One family of these GEFs is comprised of the Ras guanine-nucleotide releasing proteins (RasGRPs) that can activate Ras or Rap, of which there are four in humans. GEFs activate Ras-family members by triggering the release of GDP and its replacement by GTP. The N-terminal portion of the RasGRPs contains the catalytic module that is common to other GEFs that operate on Ras-family members. This module consists of a Ras-exchanger motif (REM) domain followed by a Cdc25 domain. As first revealed by structural analysis of the Ras-specific GEF Son-of-Sevenless (SOS), the Cdc25 domain interacts with Ras and is responsible for nucleotide release, and the REM domain provides structural support for the Cdc25 domain.

We found that RasGRP1 and RasGRP4 are specific for Ras, whereas RasGRP2 has a clear preference for Rap1B. Instead, we determined the structures of the catalytic modules of two other members of the family, RasGRP4 and RasGRP2, bound to nucleotide-free HRas and Rap1B, respectively. Comparison of the structures of the RasGRP4:HRas and RasGRP2:Rap1B complexes show that nucleotide-free HRas and Rap1B are bound in a similar fashion to the two RasGRP proteins, and that the binding mode is similar to that seen in SOS:HRas and Epac2:Rap1B complexes. An intriguing aspect of the RasGRP2:Rap1B structure is that the linker connecting the REM domain to the Cdc25 domain (REM-Cdc25 linker) is ordered in its entirety. In the structure of RasGRP2:Rap1B, the REM-Cdc25 linker runs along the surface of helix J, and wraps around it by forming an α helix. The sequence of the linker is conserved between RasGRP1 and RasGRP2, but is drastically different in RasGRP4. The structure of the linker as visualized in the RasGRP2 structure is of potential functional importance, because it is inconsistent with adoption of the autoinhibited structure of RasGRP1 that we have defined earlier (compare Figure 6A and B with Figure 6E). A prominent feature in the active RasGRP2 structure is the formation of an ion-pair between Arg 131, in the REM-Cdc25 linker and Asp 177 in the Cdc25 domain (Arg 181 and Asp 228 in RasGRP1). This salt bridge and the position of the REM-Cdc25 linker reinforces the active conformation of RasGRP and is incompatible with the autoinhibited conformation. The positioning of the REM-Cdc25 linker in the RasGRP2:Rap1B complexes places the side chain of Thr 134 close to the side chains of the positively charged Lys 172 and Arg 195 in the Cdc25 domain, which provides a possible explanation for the activating effect of phosphorylation of the threonine residue, which adds a negative charge. The high sequence conservation of the REM-Cdc25 linker between RasGRP1 and RasGRP2 suggests that the linker might adopt the same conformation in the active states of both molecules.

>[8x]SNAMAGTLDLDKGCTVEELLRGCIEAFDDSGKVRDPQLVRMFLMMHPWYIPSSQLAAKLLHIYQQSRKDNSNSLQVKTCHLVRYWISAFPAEFDLNPELAEQIKELKALLDQEGNRRHSSLIDIDSVPTYKWKRQVTQRNPVGQKKRKMSLLFDHLEPMELAEHLTYLEYRSFCKILFQDYHSFVTHGCTVDNPVLERFISLFNSVSQWVQLMILSKPTAPQRALVITHFVHVAEKLLQLQNFNTLMAVVGGLSHSSISRLKETHSHVSPETIKLWEGLTELVTATGNYGNYRRRLAACVGFRFPILGVHLKDLVALQLALPDWLDPARTRLNGAKMKQLFSILEELAMVTSLRPPVQANPDLLSLLTVSLDQYQTEDELYQLSLQREPRSKSSPTS;>GAMREYKLVVLGSGGVGKSALTVQFVQGIFVEKYDPTIEDSYRKQVEVDAQQCMLEILDTAGTEQFTAMRDLYMKNGQGFALVYSITAQSTFNDLQDLREQILRVKDTDDVPMILVGNKCDLEDERVVGKEQGQNLARQWNNCAFLESSAKSKINVNEIFYDLVRQINR[8x]> MKSSHHHHHHENLYFQSNAQRWRSDGRCGPNYPAPDANPGECNPHAVDHCCSEWGWCGRETSHCTCSSCVDYSAGGGSSGGSTVVVSSSGTCPRIVSKS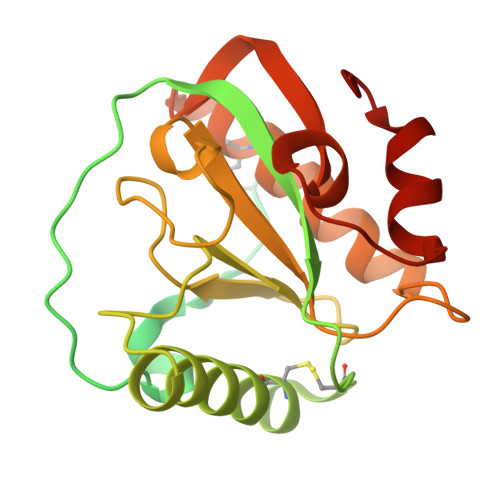EWGSRATNYNVFLSLPVPKVVIHHSAGATCSTQSSCSLQVRNIQNYHMDGRGYSDIGYNFLVGNDGNVYEGRGWDRRGAHALNVNTESIGICFMGDFTSQKPTASAIAAAKSLISCGVSLGKIRSGYSLYGHRDVGSTACPGNLLYDDIKSWGRYVG Olfactomedins (OLFs), modular proteins containing an OLF domain that are predominantly expressed in neural tissues, are involved in fundamental processes of cell growth, cell signaling and cell adhesion. High-resolution crystal structures of the ∼30 kDa five-bladed β-propeller OLF domain are available for four subfamily members: olfactomedin-1, latrophilin, myocilin and gliomedin. While the folds are nearly indistinguishable [Fig. 1(a)], one difference is the presence or absence of a heptacoordinate calcium ion bound in the central internal solvent-filled cavity of the β-propeller [Fig. 1(b)]. To survey the OLF triads for calcium binding and to test whether calcium binding can be reverted by simultaneously altering Asn428 to an acidic Asp or Glu, we replaced the triad Asp–Asn–Asp with Asp–Glu–Ser, Asp–Asp–His and Asp–Glu–Lys via site-directed mutagenesis of Asn428 and Asp478.

Asp–Asp–His is the second-ranked triad in Nematoda. For myoc-OLFN428D/D478H, nearly all residues were traced; residues 291–292 in monomer A and residues 292–293 in monomer B could not be traced, although several loops in both molecules were difficult to model, suggesting overall loop flexibility for this variant as well. The main and side chains of Lys503 and the carboxy-terminus form several hydrogen-bonding interactions with residues 242–243. The far N-terminal region adopts an extended loop conformation, forming crystal contacts [Supplementary Fig. S3(d)] with (i) a side helix of one symmetry-related monomer A, (ii) the outermost strand of blade E in a second symmetry-related monomer A and (iii) two loops (439–446 and 468–475) of a symmetry-related monomer B. For myoc-OLFN428E/D478K the difference upon the addition of calcium is within the error of DSF (±2°C), suggesting that myoc-OLFN428E/D478K cannot bind calcium; for myoc-OLFN428D/D478H a marginal stabilization was observed with calcium, suggesting weak if any calcium binding. For myoc-OLFN428D/D478H, the coordination environment is most consistent with a pentacoordinated metal ion, assigned in our model as Na+; consistent with DSF results, this metal ion does not appear to be a well ordered Ca2+, as poor thermal factors and/or occupancies result when this metal is replaced with Ca2+ (not shown). In sum, unlike myoc-OLFWT, neither myoc-OLFN428D/D478H nor myoc-OLFN428E/D478S copurifies with a fully occupied Ca2+, but both the Nematoda triad Asp–Asp–His and the Arthropoda triad Asp–Glu–Ser appear to be able to support metal-ion binding, perhaps in certain bio­logical contexts.

>LKESPSGYLRSGEGDTGCGELVWVGEPLTLRTAETITGKYGVWMRDPKPTYPYTQETTWRIDTVGTDVRQVFEYDLISQFMQGYPSKVHILPRPLESTGAVVYSGSLYFQGAESRTVIRYELNTETVKAEKEIPGAGYHGQFPYSWGGYTDIDLAVDEAGLWVIYSTDEAKGAIVLSKLNPENLELEQTWETNIRKQSVADAFIICGTLYTVSSYTSADATVNFAYDTGTGISKTLTIPFKNRYKYSSMIHYNPLEKKLFAWDNLNMVTYDIKLSKM[2x]>[2x]MENQLTKSVEERTFQYQDSLPSLPVPALEESLKKYLESVKPFANEDEYKKTEEIVQKFQEGAGKRLHQKLLERARGKRNWLEEWWLNVAYLDVRIPSQLNVNFVGPCPHFEHYWPAREGTQLERGSMMLWHNLNYWQLLRREKLPVH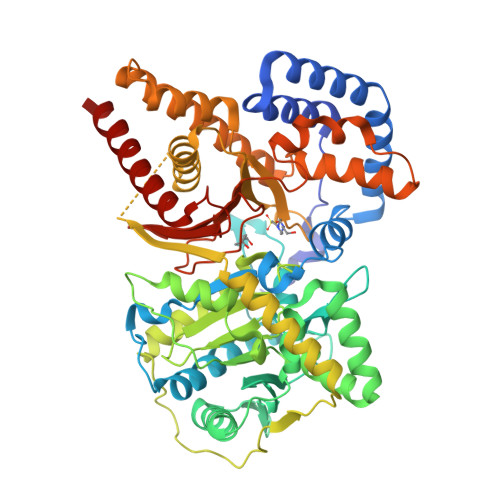KSGNTPLDMNQFRMLFSTCKVPGITRDSIMNYFKTESEGHCPTHIAVLCRGRAFVFDVLHEGCLITPPELLRQLTYIHKKCSNEPVGPSIAALTSEERTRWAKAREYLISLDPENLTLLEKIQTSLFVYSIEDSSPHATPEEYSQVFEMLLGGDPSVRWGDKSYNLISFANGIFGMCCDHAPYDAMVMVNIAHYVDERVLETEGRWKGSEKVRDIPLPEELVFTVDEKILNDVSQAKAQHLKAASDLQIAASTFTSFGKKLTKEEALHPDTFIQLALQLAYYRLHGRPGCCYETAMTRYFYHGRTETVRSCTVEAVRWCQSMQDPSASLLERQQKMLEAFAKHNKMMKDCSHGKGFDRHLLGLLLIAKEEGLPVPELFEDPLFSRSGGGGNFVLSTSLVGYLRVQGVVVPMVHNGYGFFYHIRDDRFVVACSSWRSCPETDAEKLVQMIFHAFHDMIQLMNTAHL>LGNFSQACYNSAIQGSVLTSTCIRTNGGYNTSSYDLNSVIENVDGSLKWQGSNFIETCRNTQLAGSSELAAECKTRAQQFVSTKINLDDHIAAIDGTLKYELEH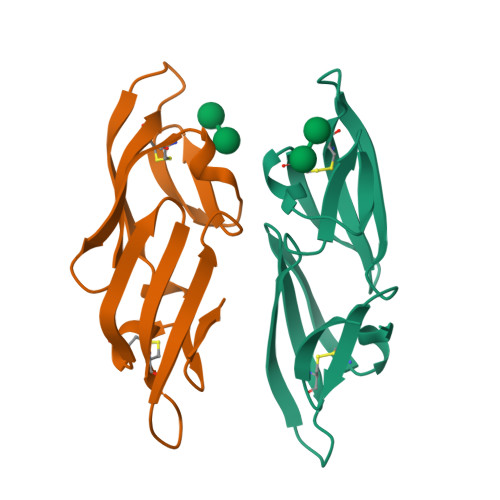HHHHH[2x]2-[4-(AMINOMETHYL)-2-CHLOROPHENOXY]-5-PYRIDIN-2-YLPHENOL | C18 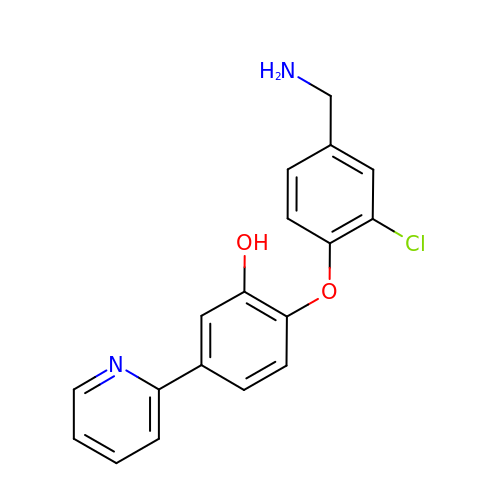H15 Cl N2 O2 | ANDLXIQDWFGHEE-UHFFFAOYSA-N> MEFLVEDLGLVPYGEAWAYQKRVHREVVAGNRPPTLLLLEHPRVITLGRKATGENLLFPESWYRENGFELYWVERGGDVTYHGPGQLVGYPIFPVGREVRRFLRQIEEAIVRVAAGYGISAYPTPGYAGVWVGEDKLCAIGVAVKEGVSFHGFALNVNTDLNDFTVIVPCGLKGKGVTSLEKLLGRKVPMEEAKARVVAAFAEVFGLRP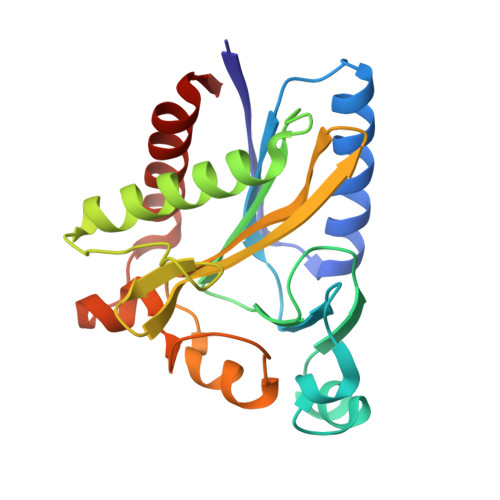V>AQDMVSPPPPIADEPLTVNTGIYLIECYSLDDKAETFKVNAFLSLSWKDRRLAFDPVRSGVRVKTYEPEAIWIPEIRFVNVENARDADVVDISVSPDGTVQYLERFSARVLSPLDFRRYPFDSQTLHIYLIVRSVDTRNIVLAVDLEKVGKNDDVFLTGWDIESFTAVVKPANFALEDRLESKLDYQLRISRQYFSYIPNIILPMLFILFISWTAFWSTSYEANVTLVVSTLIAHIAFNI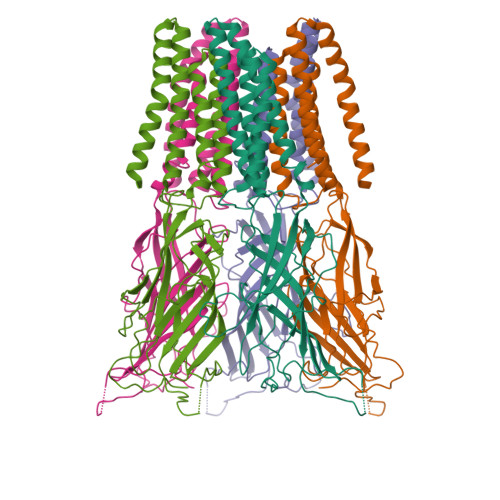LVETNLPKTPYMTYTGAIIFMIYLFYFVAVIEVTVQHYLKVESQPARAASITRASRIAFPVVFLLANIILAFLFFGF[5x]> GU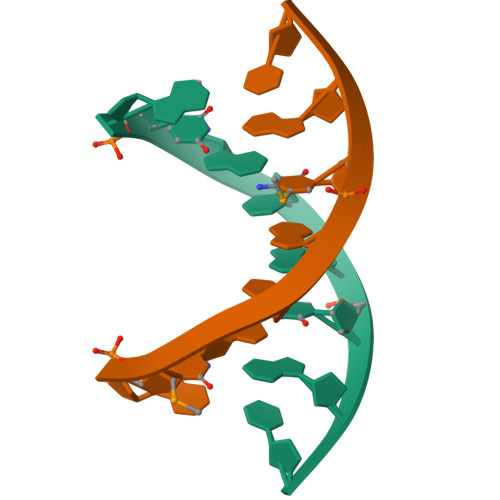GTAUAC>[4x]MLKQVEIFTDGSCLGNPGPGGYGAILRYRGREKTFSAGYTRTTNNRMELMAAIVALEALKEHCEVILSTDSQYVRQGITQWIHNWKARGWKTADKKPVKNVDLWQRL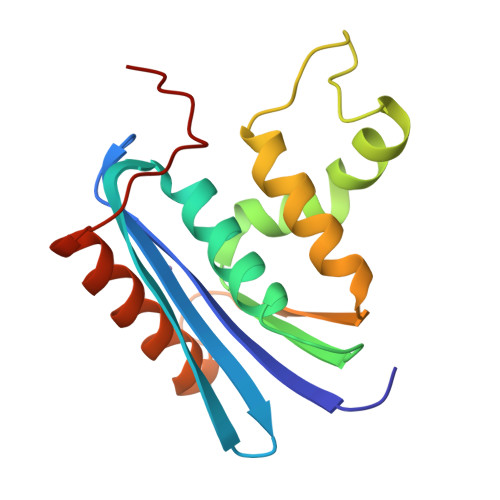DAALGQHQIKWEWVKGHAGHPENERCAELARAAAMNPTLEDTGYQVEV> MPVFHTRTIESILEPVAQQISHLVIMHEEGEVDGKAIPDLTAPVAAVQAAVSNLVRVGKETVQTTEDQILKRDMPPAFIKVENACTKLVQAAQMLQSDPYSVPARDYLIDGSRGILSGTSDLLLTFDEAEVRKIIRVCKGILEYLTVAEVVETMEDLVTYTKNLGPGMTKMAKMIDERQQELTHQEHRVMLVNSMNTVKELLPVLISAMKIFVTTKNSKNQGIEEALKNRNFTVE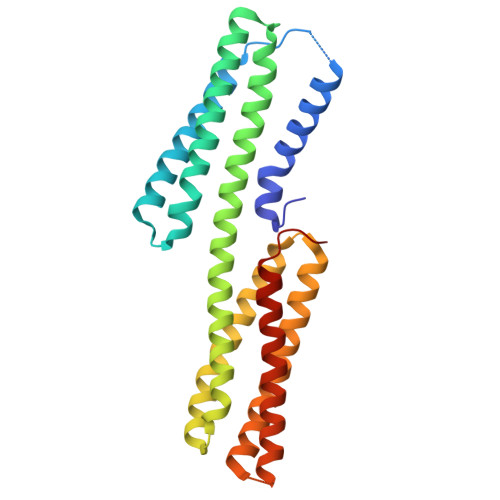KMSAEINEIIRVLQLTSWDEDAW> GSHMGTRDDEYDYLFKVVLIGDSGVGKSNLLSRFTRNEFNLESKSTIGVEFATRSIQVDGKTIKAQIWDTAGLERYRAITSAYYRGAVGALLVYDIAKHLTYENVERWLKELRDHADSNIVIMLVGNKSDLRHLRAVPTDEARAFAEKNGLSFIETSALDSTNVEAAFQTILTEIYRIVSQKQMSDRRENDMSPSNNVVPIHVPPTT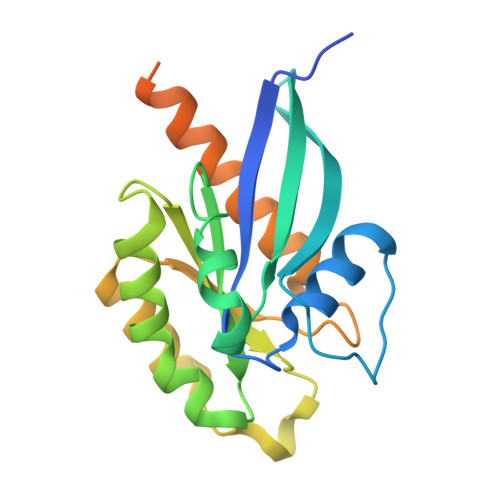ENKPKVQCCQNI> GNNVVVLGTQWGDEGQGKIVDLLTERAKYVVRYQGGHNAGHTLVINGEKTVLHLIPSGILRENVTSIIGNGVVLSPAALMKEMKELEDRGIPVRERLLLSEACPLILDYHVALDNAREKARGAKAIGTTGRGIGPAYEDKVARRGLRVGDLFDKETFAEKLKEVMEYHNFQLVNYYKAEAVDYQKVLDDTMAVADILTSMVVDVSDLLDQARQRGDFVMFEGAQGTLLDIDHGTYPYVTSSNTTAGGVATGSGLGPRYVDYVLGILKAYSTRVGAGPFPTELFDETGEFLCKQGNEFGATTGRRRRTGWLDTVAVRRAVQLNSLSGFCLTKLDVLDGLKEVKLCVAYRMPDGREVTTTPLAADDWKGVEPIYETMPGWSESTFGVKDRSGLPQAALNYIKRIEELTGVPIDIISTGPDRTE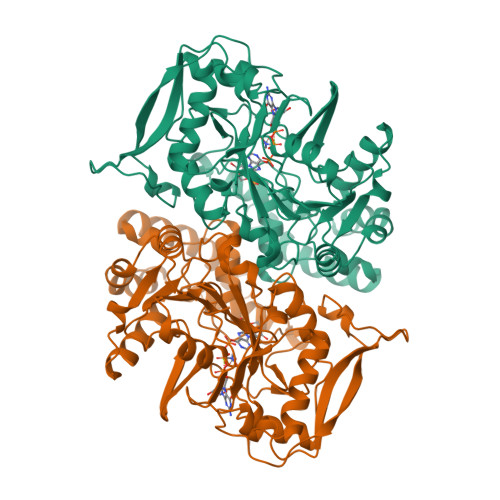TMILRDPFDA>[2x]MAKQATMKNAALKQLTKDADEILHLIKVQLDNLTLPSCPLYEEVLDTQ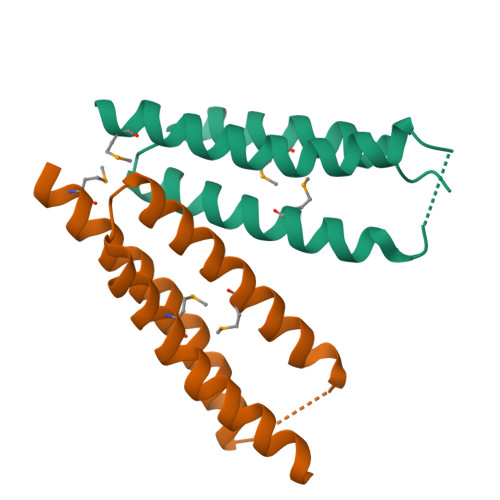MFGLQKEVDFAVKLGLVDREDGKQIMLRLEKELSKLHEAFTLV>GMARCERLRGAALRDVLGQAQGVLFDCDGVLWNGERIVPGAPELLQRLARAGKNTLFVSNNSRRARPELALRFARLGFAGLRAEQLFSSALCAARLLRQRLPGPPDASGAVFVLGGEGLRAELRAAGLRLAGDPGEDPRV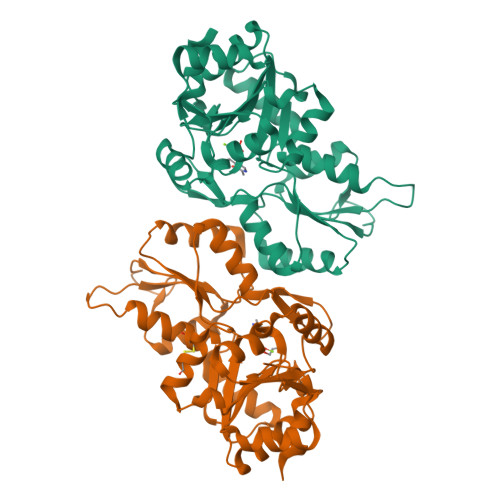RAVLVGYDEQFSFSRLTEACAHLRDPDCLLVATDRDPWHPLSDGSRTPGTGSLAAAVETASGRQALVVGKPSPYMFQCITEDFSVDPARTLMVGDRLETDILFGHRCGMTTVLTLTGVSSLEEAQAYLTAGQRDLVPHYYVESIADLMEGLED[2x]>MSDAAPSLSNLFYDPTYNPGQSTINYTSIYGNGSTITFDELQGLVNSTVTQAIMFGVRCGAAALTLIVMWMTSRSRKTPIFIINQVSLFLIILHSALYFKYLLSNYSSVTYALTGFPQFISRGDVHVYGATNIIQVLLVASIETSLVFQIKVIFTGDNFKRIGLMLTSISFTLGIATVTMYFVSAVKGMIVTYNDVSATQDKYFNASTILLASSINFMSFVLVVKLILAIRSRRFLGLKQFDSFHILLIMSCQSLLVPSIIFILAYSLKPNQGTDVLTTVATLLAVLSLPLSSMWATAANNASKTNTITSDFTTSTDRFYPGTLSSFQTDSINNDAKSSLRSRLYDLYPRRKETTSDKHSERTFVSETADDIEKNQFYQLPTPTSSKNTRIGPFADASYKEGEVEPVDMYTPDTAADEEARKFWTEDNNNL[2x];>[2x]HALQLKPGQPLY

The fungal class D1 G-protein-coupled receptor (GPCR) Ste2 has a different arrangement of transmembrane helices compared with mammalian GPCRs and a distinct mode of coupling to the heterotrimeric G protein Gpa1–Ste2–Ste181. Ste2 is a homodimer that can couple to two G proteins simultaneously and its dimer interface is formed by the N terminus, extracellular loop 1 (ECL1) and transmembrane helices H1 and H7. Here we determined structures of Saccharomyces cerevisiae Ste2 in the absence of G protein in two different conformations bound to the native agonist α-factor, bound to an antagonist and without ligand. Activation of Ste2 requires both the removal of a blockage from the G protein coupling site (H7) and formation of the binding site primarily through the inward movement of H6.

The antagonist is a mutated form of α-factor with Trp1 deleted and the W3A mutation added; conversion of Met12 to Nle does not affect signalling but makes the peptide more resistant to oxidation. The antagonist adopts the same hairpin shape as α-factor in the orthosteric binding pocket, but makes contacts with fewer residues in the receptor (20 compared with 32 in Ste2–Ag–G). The structure of the antagonist N terminus bound to Ste2 is linear, with His2 forming a hydrogen bond with Asn2055x29 on H5 and Ala3 interacting with Thr274ECL3 in ECL3. Upon antagonist binding, the side chains of Phe2045x28 flip inwards by 180˚ (7 Å inward shift of the Cα atom). Lys2025x26 has to flip in the opposite direction to prevent it clashing with the ligand, although there is only weak density for the side chain in Ste2–Ant because it extends into the detergent micelle. In the Ste2–Ant state, the receptor transitions from density maps that lack signal for the N terminus of the antagonist peptide to maps where this region becomes discernible, whereas the C terminus of the peptide is clearly visible. The intracellular end of H6 in Ste2–Ant is kinked outward away from the receptor core by 38˚ (12 Å shift at Cα Ser2436x35) compared with its position in Ste2–Ag–G, and this section is also rotated by 170° along the helix axis. By contrast, in Ste2–Ant, H7 is kinked in towards the receptor core at an angle that differs by 47° from the active state and the residues Ala2967x56–Ser3037x63 form a random coil. The position of the intracellular end of H7 in Ste2–Ant overlaps with the position of the α5 helix1 of the α-subunit Gpa1 in Ste2–Ag–G and thus sterically blocks G protein coupling. Notably, two putative sterol molecules reside at the kink in H7 in the inactive states of Ste2, but not in the active states; the sterol ergosterol is known to be important for Ste2 function.> ATAAEIAALPRQKVELVDPPFVHAHSQVAEGGPKVVEFTMVIEEKKIVIDDAGTEVHAMAFNGTVPGPLMVVHQDDYLELTLINPETNTLMHNIDFHAATGALGGGGLTEINPGEKTILRFKATKPGVFVYHCAPPGMVPWHVVSGMNGAIMVLPREGLHDGKGKALTYDKIYYVGEQDFYVPRDENGKYKKYEAPGDAYEDTVKVMRTLTPTHVVFNGAVGALTGDKAMTAAVGEKVLIVHSQANRDTRPNLIGGHGDYVWATGKFNTPPDVDQETWFIPG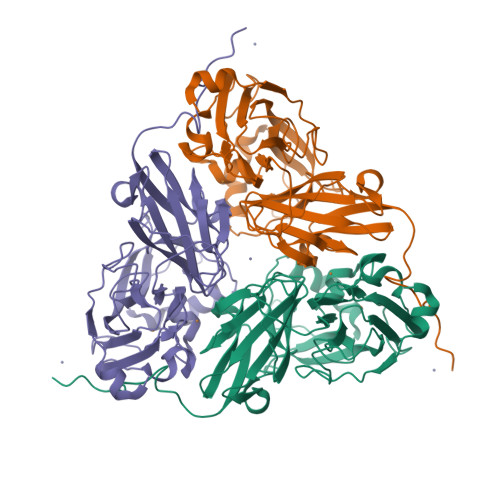GAAGAAFYTFQQPGIYAYVNHNLIEAFELGAAAHFKVTGEWNDDLMTSVLAPSGTIEGR> SGIVQQQNNLLRAIEAQQHLLQLTVWGIKQLQAASGGRGG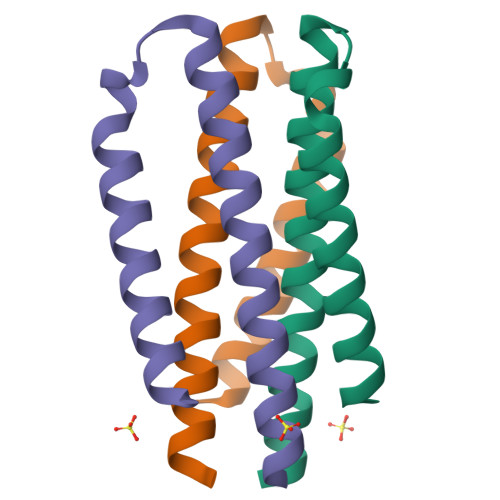WMEWDREINNYTSLIHSLIEESQNQQEK>[4x]MSRPRILVPGKINPRVLERLPEMFETVRIERADAALVTADMRDVSGIAVSGKLPVPLMDAFPSLEIVANFGVGYDGVDVSRAAARGIVVTNTPDVLTEEVADTAIGLLLNTLRLLPQAEQWLRQGRWVREGAFPLSPLSLRGRTVGLFGL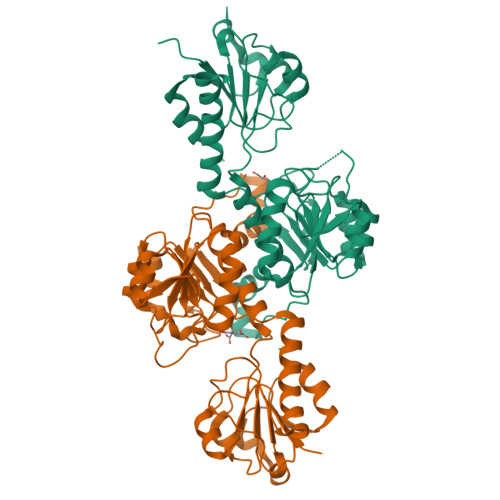GRIGLAIARRLEAFGVSIAYHTRTPREGLGFTYHPTLVGMAEAVDTLIVIVPGTASTLKAVNADVLSALGPKGVLINVGRGSTVDEAALVTALQNGTIAGAGLDVFENEPNVPEALLSFPNVSLLPHVASASVVTRNAMSDLVVDNLKAWFSTGEALTPVAETPFRRRAIQN>[6x]GPLGSPEFAEKESHASCSC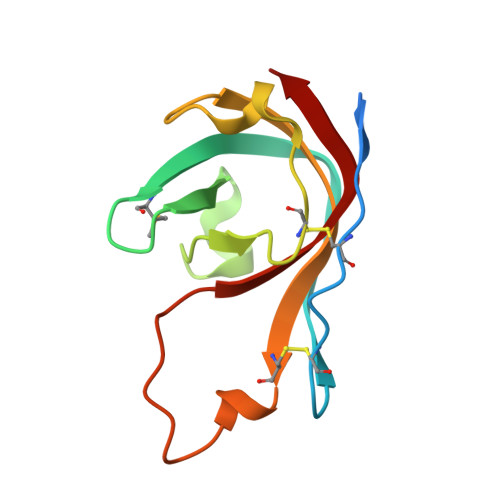ECVEEKIPIVTLKNENAHFRYMKRRNDFALEIENKELVRGLYLIPRGCDIPKKYKEDGLPVIISGEVFDCSEYIKPWIKRDPVYFIKLSTIKKK> MLDEALMPKHIALIMDGNRRWAKDKGLDVSEGHKHLFPKLKEICDISSKLGIQVITAFAFSTENWKRAKGEVDFLMQMFEELYDEFS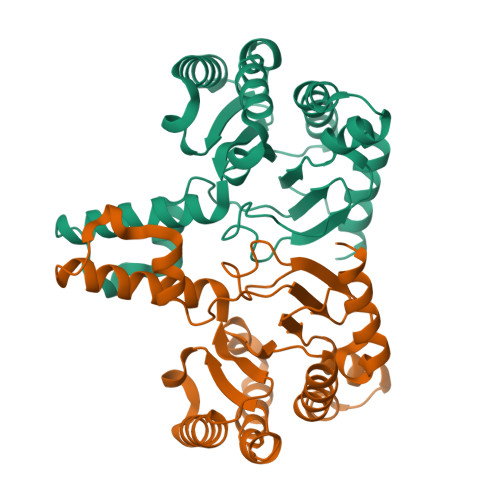RSGVRVSIIGCKTDLPMTLQKCIALTEETTKGNKGLHLVIALNYGGYYDILQATKSIVNKAMNGLLDVEDINKNLFDQELESKCPNPDLLIRTGGDQRVSNFLLWQLAYTEFYFTKTLFPDFGEEDLKEAIINFQQRHRRFGGHTY> GAMAGQGDGSVIELGEQTVVATAQEETKQAPGVSIITAEDIAKRPPSNDLSQIIRTMPGVNLTGNSSSGQRGNNRQIDIRGMGPENTLILVDGKPVSSRNSVRYGWRGERDSRGDTNWVPADQVERIEVIRGPAAARYGNGAAGGVVNIITKQAGAETHGNLSVYSNFPQHKAEGASERMSFGLNGPLTENLSYRVYGNIAKTDSDDWDINAGHESNRTGKQAGTLPAGREGVRNKDIDGLLSWRLTPEQTLEFEAGFSRQGNIYTGDTQNTNSNNYVKQMLGHETNRMYRETYSVTHRGEWDFGSSLAYLQYEKTRNSRINEGLAGGTEGIFDPNNAGFYTATLRDLTAHGEVNLPLHLGYEQTLTLGSEWTEQKLDDPSSNTQNTEEGGSIPGLAGKNRSSSSSARIFSLFAEDNIELMPGTMLTPGLRWDHHDIVGDNWSPSLNLSHALTERVTLKAGIARAYKAPNLYQLNPDYLLYSRGQGCYGQSTSCYLRGNDGLKAETSVNKELGIEYSHDGLVAGLTYFRNDYKNKIESGLSPVDHASGGKGDYANAAIYQWENVPKAVVEGLEGTLTLPLADGLKWSNNLTYMLQSKNKETGDVLSVTPRYTLNSMLDWQATDDLSLQATVTWYGKQKPKKYDYHGDRVTGSANDQLSPYAIAGLGGTYRLSKNLSLGAGVDNLFDKRLFRAGNAQGVV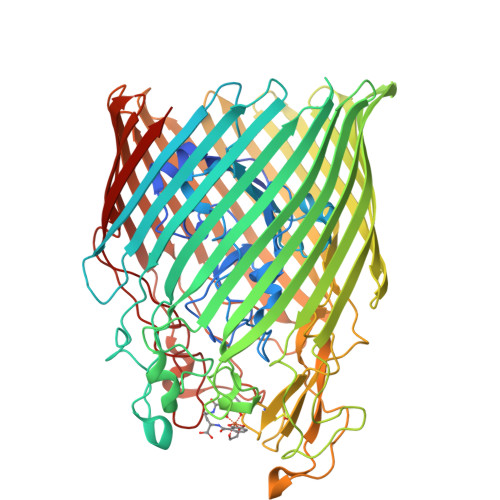GIDGAGAATYNEPGRTFYTSLTASF>MTSAEMTSPNNNSEHQAIAKMRTMIEGFDDISHGGLPIGRSTLVSGTSGTGKTLFSIQFLYNGIIEFDEPGVFVTFEETPQDIIKNARSFGWDLAKLVDEGKLFILDASPDPEGQEVVGGFDLSALIERINYAIQKYRARRVSIDSVTSVFQQYDASSVVRRELFRLVARLKQIGATTVMTTERIEEYGPIARYGVEEFVSDNVVILRNVLEGERRRRTLEILKLRGTSHMKGEYPFTITDHGINIFPLGAMRLTQRSSNVRVSSGVVRLDEMCGGGFFKDSIILATGATGTGKTLLVSRFVENACANKERAILFAYEESRAQLLRNAYSWGMDFEEMERQNLLKIVCAYPESAGLEDHLQIIKSEINDFKPARIAIDSLSALARGVSNNAFRQFVIGVTGYAKQEEITGLFTNTSDQFMGAHSITDSHISEITDTIILLQYVEIRGEMSRAINVFKMRGSWHDKAIREFMISDKGPDIKDSFRNFERII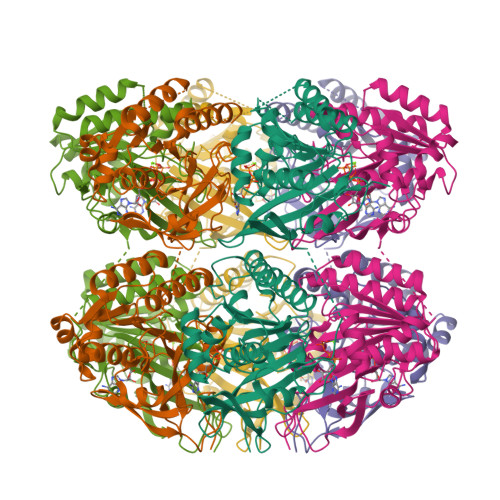SGSPTRITVDEKSELSRIVRGVQEKGPES[2x]>[14x]MNLIPTVIETTNRGERAYDIYSRLLKDR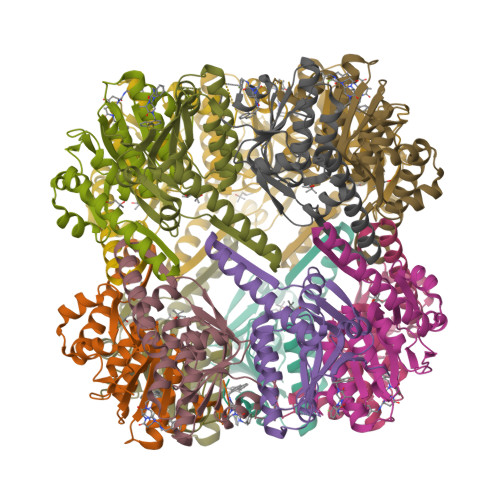IIMLGSQIDDNVANSIVSQLLFLQAQDSEKDIYLWINSPGGSVTAGFAIYDTIQHIKPDVQTICIGMAASMGSFLLAAGAKGKRFALPNAEVMIHQPLGGAQGQATEIEIAANHILKTREKLNRILSERTGQSIEKIQKDTDRDNFLTAEEAKEYGLIDEVMVPETKLEHHHHHH> QPDPKLDELNK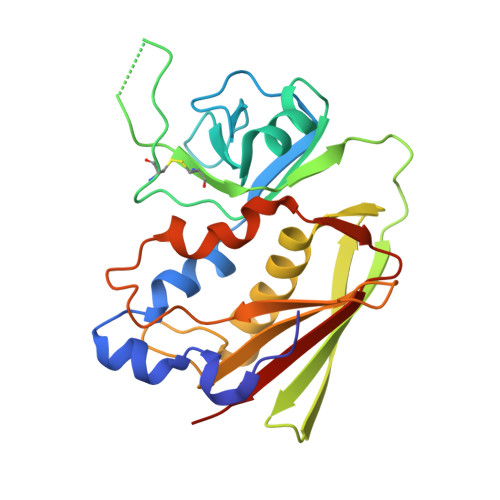VSDYKSNKGTMGNVMNLYMSPPVEGRGVINSRQFLSHDLIFPIEYKSYNEVKTELENTELANNYKGKKVDIFGVPYFYTCIIPKSEPDINQNFGGCCMYGGLTFNSSENERDKLITVQVTIDNRQSLGFTITTNKNMVTIQELDYKARHWLTKEKKLYEFDGSAFESGYIKFTEKNNTSFWFDLFPKKELVPFVPYKFLNIYGDNKVVDSKSIKMEVFLNTHHHHHHH The Vesivirus feline calicivirus (FCV) belongs to the family of Caliciviridae which carry a positive strand RNA genome which is enclosed in a capsid composed of 180 copies of the major capsid protein forming an icosahedral T = 3 shell. In contrast to the other genera, Vesivirus VP1 is synthesized as a precursor (668 residues for FCV) which is processed by the viral protease into a 124 res. leader peptide and the 544 res. Feline Junctional Adhesion Molecule-A (fJAM-A) was identified as a cellular receptor for FCV. We observed that the majority of the FCV VLPs obtained from the expression of VP1 in the baculovirus system are small sub-viral particles made of 60 subunits with T = 1 symmetry different from viral capsids.

The crystal belongs to the cubic space group P213 with a cell parameter of 358.3 Å. It became obvious that here was no electron density for the N-terminal 37 residues which correspond roughly to the NTA domain. In the T = 3 capsid these residues are involved in inter-subunit contacts interlocking the shell of VP1 capsid proteins. VP1 forms a closely packed shell without any significant openings. The particle has an outer biggest dimension of 295 Å at the position of the spikes, whereas the shell extends only to a diameter of 185 Å. There is no indication that the structures of the S and the P domains differ from the corresponding ones from the T = 3 crystal structure of the viral particle. But in order to adapt to the T = 1 shell, the relative positions of the S and P domains change from the ones observed in the T = 3 structure. The structural adaptation to the two types of particles involves a hinge movement between the VP1 S and P domains resulting in a slight rotation of the spike around its 2-fold axis which is combined with a translation of the P domain relative to the S domain. A comparison of these different oligomers in the T = 1 and the T = 3 structures confirm the conservation of the contacts within the oligomers. The conservation of the arrangement of the VP1 capsomers around the 2-fold, the 5-fold and the 3-fold icosahedral axes between the native T = 3 virus particles and the T = 1 VLPs shows that the antigenicity of the protein is conserved and that the use of the T = 1 particles for vaccination is a pertinent approach.

>MADDGSITAPEQGTLVGGVIAEPSAQMSAAADMATGKSVDSEWEAFFSFHTSVNWSTSETQGKILFKQALGPLLNPYLTHLAKLYVAWSGSIDVRFSISGSGVFGGKLAAIVVPPGVDPVQSTSMLQYPHVLFDARQVEPVVFTIPDLRSTLYHLMSDTDTTSLVIMIYNDLINPYANDANSSGCIVTVETKPGSDFKFHLLKPPGSMLTHGSVPSDLIPKSSSLWIGNRYWTDITDFVIRPFVFQANRHFDFNQETAGWSTPRFRPITVTISQKGGEKLGIGIATDFIVPGIPDGWPDTTIPSKLTPAGDYAVTTSNGTDITTPREYDSANEIVNNTNFKSMYICGALQRAWGDKKISNTAFITTATVEGNNLEPSNVINPTKIAVFQDNHVNRDVQTSDVTLALLGYTGIGEEAIGADRDKVVRISVLPETGARGGNHPIFYKNTVKLGYVIRSIDVFNSQILHTSRQLSLNNYLLPPDSFAVYRIIDANGSWFDIGIDSDGFSFVGVSNIGKLEFPLSASYMGIQLAKIRLASNIRSTMTKL[20x]(2~{S})-2-[[(2~{S})-6-[(4-fluorophenyl)methylamino]-1-oxidanyl-1,6-bis(oxidanylidene)hexan-2-yl]carbamoylamino]pentanedioic 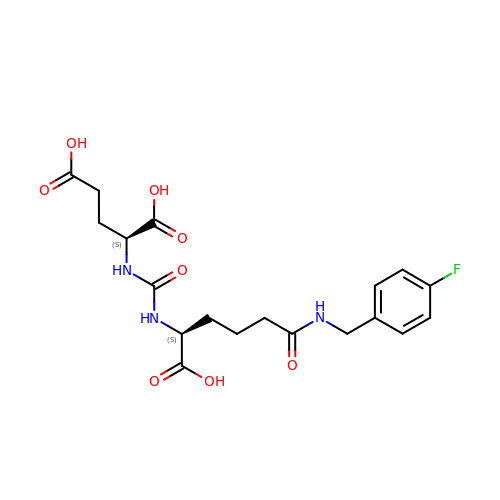acid | C19 H24 F N3 O8 | ZCBCSGACSCSXNO-KBPBESRZSA-N propan-2-yl (R)-dodec-11-en-1-ylphosphonofluoridate | C15 H30 F O2 P | 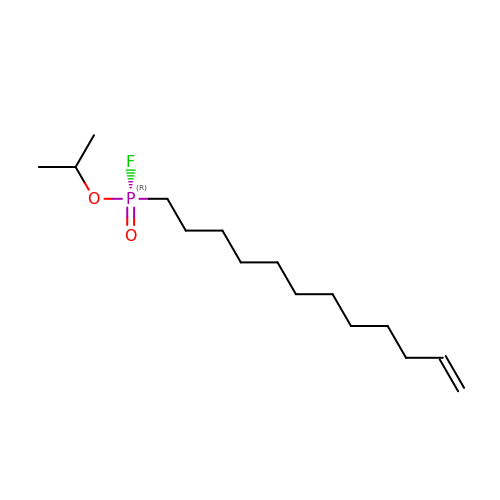HAGAHLUSUUTRJV-LJQANCHMSA-N> MGTISSAIINHAFLQNTVMKNCNYKRKRRERDWDCNTKKDVCIPDRRYQLCMKELTNLVNNTDTNFHRDITFRKLYLKRKLIYDAAVEGDLLLKLNNYRYNKDFCKDIRWSLGDFGDIIMGTDMEGIGYSKVVENNLRSIFGTASTAATSRTSWWNESKAQIWTAMMYSVKKRLKGNFIWICKLNVAVNIEPQIYRWIREWGRDYVSELPTEVQKLKEKCDGKINYTDKKVCKVPPCQNACKSYDQWITRKKNQWDVLSNKFISVKNAEKVQTAGIVTPYDILKQELDEFNEVAFENEINKRDGAYIELCVCSVEEAKKNTQEVVT

P. vivax Duffy Binding Protein (DBP) is a surface protein that the parasite uses to invade host red blood cells and is a leading vaccine candidate. DBP is a member of the Duffy binding-like erythrocyte binding protein (DBL-EBP) family, and binds DARC through a conserved cysteine-rich DBL domain known as region II (DBP-II). DBP-II engages DARC through a multimeric assembly mechanism where two DBP-II domains initially bind one DARC to form a heterotrimer that rapidly recruits a second DARC to form a heterotetramer. Consistent with this view, the most polymorphic region, identified as the DEK epitope, is positioned immediately adjacent to the conserved DARC-binding groove.

To overcome this inherent deficiency of DBP as an immunogen, a novel synthetic DBP-II antigen termed DEKnull was engineered where the polymorphic residues that comprise the DEK epitope were mutated to amino acids not usually present. We obtained the crystal structure of the DEKnull antigen to a resolution of 2.1 Å. DEKnull maintains the overall fold and conserved disulfide bonding patterns of a DBL domain similar to that found in P. vivax DBP Sal1, from which DEKnull is derived. DEKnull also retains the characteristic three sub-domain architecture of DBL domains with critical intra-domain disulfide bonding patterns. All cysteines in DEKnull are involved in disulfide bonding and are structurally conserved with Sal1 DBP-II. Alignment of DEKnull and Sal1 DBP-II structures shows minimal differences with an overall root-mean-square (r.m.s.) deviation of 0.435 Å, indicating there is minimal differences overall between the native and engineered domains. S2 alignment has a r.m.s. deviation of 0.288 Å, and the only change is the region comprising K366 to I376, which is now structured in DEKnull as compared to Sal1 DBP-II. Strikingly, the DEKAQQRRKQ polymorphic stretch within S2 overlaps well between DEKnull and Sal1 DBP-II. Alteration of these amino acids to ASTAATSRTS had no affect on the secondary structure nor do they shift peptide backbone Cαs. The dimerization and DARC binding surfaces overlap well with the parental Sal1 DBP-II; there is no allosteric change to secondary structure or peptide backbone Cαs, retaining the conformational shape of protective targets.The mitochondrial ATP synthase is a membrane protein complex that generates most of the ATP in eukaryotic cells. The translocation of protons through the membrane-bound Fo part, mediated by subunit a, drives the rotation of a membrane-embedded c-ring and the attached central stalk, which together form the rotor. The torque of the rotor against the stator subunits induces conformational changes in the (αβ)3 headpiece, thereby triggering catalysis. To reveal how the mitochondrial ATP synthase is modulated by lipids and organised into a dimer shaping discoid cristae in Euglenozoan mitochondria, we determined the structure of the ATP synthase dimer from E. gracilis.

The mitochondrial ATP synthase dimer was purified natively from E. gracilis and subjected to cryo-EM structure determination. The atomic model of the entire 2-MDa complex contains 29 different subunits (eight newly identified) and provides a comprehensive description of a markedly distinct mitochondrial ATP synthase dimer, including a previously unseen binding mode of its natural inhibitor protein IF1. The model of the complete mitochondrial ATP synthase contains 29 different proteins, of which 14 are phylum-specific, displaying a distinct architecture, particularly in the membrane region. The interactions between the monomers are expanded, resulting in a 45° dimer angle, compared to ~100° in yeast and mammals. Our atomic model of the E. gracilis mitochondrial ATP synthase shows that in contrast to yeast, subunits a, i/j, k do not contribute to the dimer interface, which instead is formed by species- and phylum-specific subunits and extensions of apparent homologs. The extensive dimer contacts are stacked across three layers: the matrix side, the transmembrane region and the lumenal side. Thus, despite the presence of conserved Fo subunits and the contribution to their extensions to the dimer interface, the E. gracilis mitochondrial ATP synthase displays a fundamentally different dimer architecture, when compared to the yeast, mammalian and Polytomella ATP synthases, suggesting that dimer formation evolved independently in different lineages. Our unsharpened map of the ATP synthase dimer with both monomers in rotational state-1 (IF1pointing towards the C2-axis), shows a continuous density from the C-terminus of IF1. This density extends towards the dimer interface and contacts the all-β-fold formed by subunits b and d, suggesting that also in Euglenozoa both F1 complexes in the ATP synthase dimer may be inhibited by a dimeric IF1. However, in contrast to the mammalian ATP synthase, the specific binding mode of the Euglenozoan IF1 assembly links two monomers within the dimer, rather than between neighbouring dimers.

>[2x]MTAVVKNLAKLPAATSQILTNVSKLQTFHGLLEERRDKYAPLAYHTYDNLKQKTTWHPIAHAWVDEGLPVSKKEYNEYCWLKKDMQRLLPLASPFVFGIYGILPLAVWLSNDGYLPSAFSSKKDIVSKKLEWYSSYGDDLRQQVGPMLQHRLKRHLRGTLNNEHRLMLDEVTESYKEIFYSHYTGQLRDVRKCAHLRLYDGTSTVLLLTNKEPVELTSELLQKWNAIKAAKLSPEEEKKARNEALIEAYKEQELHGGPHVKHMQGYGIPADTPLLGENAKGDQYTQPPESASIPLEQLEWTGDTVFIPAEYRTEMEDWGRELTKLANQFLLLPWRFVSNAWNQRRLVSWFEEILQEDALIAKEGGVQALSDDELKVALLDRAVIRCDEELTRGDMEARYKEISWLMSLRNPFIVLAWQTGYYRSTYSPEDDLPEASILPKLNRTVLDVDVHNELAPDHPEKPLPRVHPALYPNSHLALAKEVAVLAK;>[6x]MHYAEAATPAKSAGSAVAKKHLEAKQKIGFVHGIDGTIATIAPAASKVTVPYNTVLEIAVSATNIANALVFNLEKDGSIGVILLDNISEVRSGQDVYATGSLLKIPVGFHMLGKIINPLGKEIPTGLFTKAAPLLDDTKLGLVEEMAPNIVSRQPVNYNLLTGYKVIDTLIPVGRGQRELILGDRQTGKTSIALSTILNQTKVNNEILSKNNVLSVYVSIGQRCSNVARIHRLLTEYDAMKYCTIVAATAADPAGLQYLAPYAGTTLGEEFRNSGRHILLVYDDLSKQAVSYRQISLLLRRPPGREAYPGDVFYLHSRLLERSAMMSPQKGSGSLTSLPIVETLSNDVTAYIVTNVISITDGQIYLDAKLFTGGQRPAVNIGLSVSRVGSSAQNKAMKKVGGALKMLMGEYRKMAGEQTSGSQNVSPVMIRGARCLQLFNQKGPSYFMDAIVALYAVTNGYMDDVKLQYSKFYEFLLLNKDLPVLYGQVNNKYFYMYNKNLNYFIRYFGLNHEILEPELKKYIEIHTNLFLDNYQSRMNELKSDEDLVQLKNLLYACKRTV;>MVGRMMATAPATAADVKQVGYVQQIIGAVVDVTFTDSVPPVLTALTVDAKETGTLLTMEIVQHLDTKTARCICMSSTDMLRLRTPVVNTGSQITVPVGEATLGRIFNVMGDAIDQRGPVKNKVRWPIHRKAPTLAEQSGKDEVLVTGIKVIDLILPYCKGGKIGLFGGAGVGKTVIIMELINNVAKGHGGYSVFAGVGERTREGTDLYLEMMGSKVIDLQGDSKCVLVYGQMNEPPGARARVAQTALTMAEYFRDEAGQDVLLFVDNVFRFTQANSEVSALLGRIPAAVGYQPTLAEDLGMLQERITSTVKGSITSVQAVYVPADDITDPAPATTFSHLDATTVLSRSVAEAGIYPAVEPLECASRIMDPDAIDVNHYNVAMDIVEMLTKYKELQDIIAVLGIDELSEEDKLIVDRARKVAKFMSQPFAVAEVFTGMKGYYVQLEDCVSDFGSLLMGQCDNIPEMAFYMVGGLDSVKEKAAKMAAEAAAMRERARKAAEAK[6x];>[2x]MPGGGTIRFWREKLEGYKKYHQIVKTIKMVTLAKYRQTVVRTRVRDQTLRYTRKALDAKTQDDQEVIEKSECLLYVPITTNRGSCGALNTNMVRYLQEVENPKMTIISVGKKALDAMTKVFQDTYRRTILNDMKQAMSFQFAAYVLEHMNTVPWDRAQIVYNRYHGAASQKLAIFNLPKFEDWKQKLEEDSAGDGKIEEDGLLQSLPMKTALGELEETAVEDFYNFHSCLAVLNAVSENELSEYAARIVAVENQLGNITGLMQLADYTYNKTRKELITAELLEIIGTMTAMHAGKKVGLKKTEFWK;>[2x]MRASRTLLLSVSRFMRQDPRKFFPDNGFRFFDGPEDSFGDGNIPAQIILTLTRQDEFILKQEPVAAITIRTNEGEMGVLAGHEYTVQQLAPGILEVEYEGGKKDQYVISGGFAHVNDTGVVDINTVEAVPLEEIDHEKLAKALEEARAKSQSPDEAVRIQGEIALEIFEPLEAALH;>MSWRDAGISYLRYLSIVTRCIHEVQKEGPLLTKNVRFSTIGWKSLYLDHGATKEYTAIPAELEKIPENQVAQQHHA[2x];>MQKLSRVVCNRLVRFHGTVAASAGGKRYDLFGYEVSVATGPFIEEIKKAQFYDDAGEVIVKMNLANTPPDLQTYNAVLERILNCKSKRSQPVKGENKFAAMMDILEEMDARSGIKPNAESWGYVLKELVQAGDFRLGWVCIAGMKSLGITPDQALVDANEANAAKAKAAGTDFPAYLKKAAPESFDTKAWGI[6x];>MHMRRAVSVFGRCRSLNGLRNYAVPSPKYIEIYQSDFSRNAYPLELLGGSHVDFAKLLYSFADQVENKKFEVYVEDFKKLDSIIAEKGPFWAEEKIFQSPTFQGLSEGFKFILGWIQSEGAIDRLENVRLAYKELVNEARKETTATVIVAKEPSGNDLAEIRKQVEELHKESPLKDYKLVLETKVDPSIGGGYILEVCNQVVNRSAAAAAAETAALAKASAAQVDWTSLPAAPPRPSPSAPDTLIRLLGSVVDDLADADKVEQKYGA[2x];>MAAACAVRGFTTARPMLTPNKVKVPGRKPQDEEDLTWAEADRKLTPEERYARDKQMALLDKMTSQVEELEKSHTEQKKSNKGVKAQIEAISRQLEALKAQLKE[2x];>[20x]MQRGSSITKVVRRAALARSTRNAAIAYEVTVNGANLIGAGMAASGVGVPAIGVAMCFSSYMLAAARQPNMSAKLLPYCILGFALSEALALFTLLIALLELFVFS;>[2x]MAAKTIPFVASTALGERLFAGVQKVLAAAKAPVSLVQTDAKFAPADAKYLLAEPLSAAATGELANKYGLSSKVTSGAASQFYPNSIYPSLNVEVVQNLYALSNPAFSSLSATTTKAVTVKDESAIKLAELQKETERNISSFFRDEANKSVQATLRLACDKAIKTKADKKTVMVVTKPHGDAFDDLLAQVTKSESDGRADELRNSSVSVEPTLVGNAWPKLVMFPEGVNVVVCGPNASGDQVAQLFVGIAGGTGMVAQQLVGDAVVFTSANAEDNENPTGALLAASNLLTALGHEAEAKKIAAAVAKAYTTDRILPKELPGGKADLEAFIDAVAKHASA;>MFRGFRPVLAADAVKFQTLYNVLTGKQHLKDQVPVKDCNLTAIFGASWKADLNKWFDSEYAPKLPAAERDSAKKSLDLYLKRVDLTRYTREELTTYGILACGPGKVDALTEKHLLETGKARLEELTAGLGNKDEGVNAFRKEVEQEGKYANWPAEKSKALADKVIAASP[2x];>MTHAELHLFDLDEFMQTYKRLQTRQDWLIENKCKKSRLFSYVAAVIAFTVGKSATMSDEAILAKIDPYVTSEVRVQRGAWWRSGYFTKEEVEMMTPKGPIARYYKFLLGVRRFPLKHGALSWACGFVPAWLTFTSLNHWAQNRRLNRYLTQESVFGEMARELVRGKTADEATTSVMARVEKEILGVH[2x];>[2x]MSSYTGAALAPKSERLRLAFEEKQKDHQKCIEEAKGKGLKKDELIDACAWTHRKTILALKDWFAYRPPFQDRRSKWAEYCSIRHDSGSWLGWSQKFF;>MLNSNIYIIIYGGIIMYSIMIIIQMFLYNFSNKIYIEVEINKYILSKNNIDIYWIICNCTIIIIITTLNHIINKIGIYNMIEYNICYWLIGTGLGLYISPFIVFGYKFFVYIMDLNNYSLNIYHNNNKMNDIQQIYNGTNYNDTMIFFIKDINNIFTIYRSINFFMNWLYQMIYYGVRMWLVFVLHSFSLGSFGELITVITDNNLIFNVFYIGLLGLGFILYLIVIFYLGIQIYVYISFSLSFLHSTILLFLVNYIPHYNNKSIFNTFTNKSIY[2x];>[2x]MPSTSPADKDVPMSILHTHGLSYVNWCMSLAPGLLVFEGFFRARYYRSRVPPSRTVLMNGLKMRMFSLARQQAPKIVHKPVLSPIPEHLRLVKNVAQVQIDMLKLLNAQAAK;>MMRRACRIIRPSHVRGVSGVAPTIYLRSKAALPATSTTDVRPQLYALQRFAKAQLKTATEAERAAIEADIARYQEYLDSDLEKLKQDVAEDTAKKQKLIPLLDRYPDVPIEKIPEHANVLLKKIDACLEILSKDIGEVTDAEAHEMYFETSKFQILHIYTGCVASFPEGDVPPGAVECLPGQVIRTKVNGEDVMLEIDEVDPGYQVCWFKPDVPLPENAEILWSYPYEPTAALPTGTTWEEGQANVLIPAEPTPEAAVWPPTPVTNVYAPMAEKLALKSNPELKVLFKEALLQPAKLLPLDVDYQCSHDREVVEAKRDRYLTALVEAEQAPPLPFTPDVLQLQLEHNVLKGELIDRLRALEYTIVTEQLQARLHERRLRGDVIDEWEELDYHPLVRDDTYLAIDFGDPTFGRYIWKLFPHTDGDEECMFKDTRLDVLPPQVNPLNAILAQHTAQTPVHRSLEKRLWTEVRATAVSE[2x];>MAPLYPVLSQASLYKRHFFKNIKLFHVVFYVGAPCVTFGTAAWSGSNRNSREAIFMVIEERHGWDNFKKLSSHQQGVIMQEAAQESLLARNKGELHLP[2x];>MVYTNWQSSYTRLFVSKPWMWHPLAWMTLSVGIWWKFGKESLCNERSFYIHTHPKWAPHKFHTVYNWSRDPIKWTLAEQYASIIRNTNTDIEAVLKIKLPANAN[2x];>[2x]MAFGRTRPTLSSPLVPVWNDLRALQVFTSQEYMQKRGPGFTNTLEYKLSCLNPVKWYDMMKVMPGGKAFVGTALGLALFGGWGVEFVKNISVMTKEKPPIDWNNEKLGHLTRS;>LIPVSLVDLININIIFYILLLYTLLLFFIPLFLASINYTYHYIYKYYNYNYNFINNN[2x];>MSLAKVWMYASWIPRGIPKAMANELSSAAAALAHPEAIARVAQLESQGKNPYRVARAEFWQMYLACWPYRFRNTVVEWETCKAKVLKGSVDLQDIVDLLYLLAWAYLFWILGEIYGRGSLYGYRFDGEIHRQEAQNVILYKEKEAQEMAVVMEKLEKEIQEWLKTMEQE[2x];>[2x]MPLPNAVVQGYTSVRGPKRPLDHFYGRTPLNIDTLWHWVKFPHRYDNLRFAVCFWAFLVSAHFANKKQRNLRVEWEKNMEIQKKLHPSGLWSEEQAFAAAEKLGRPKAGHPMRVFEDGYQQFDLKPKLFDPDEEAHH;>MADHNKKDVGSWASPNEHLMFFDFSSWLLVDFGKRWERWVSFKKSFLTTTRSPYWSPQFFLLTFFQLRNSNVKLCENWNWAPKGDDFNLLHNSAAEPFGRDLKAHLEREAGAKHHH[2x];>[2x]MGGDAHAAPAEKPDPALDATKALPKALEEVEFFQSYAVRRKTGFHLFNRATGSPTIVGPMFYNLYNFVRIGRVSKYVCWLSLPLVFQRMWMKNRATGMEYDIDLENYAPFEAKKNPMHGH;>[2x]MSLPTFFLAPPLTEPFRARHRRKCIEKKDTFFQCLDKNKNETEPCEVEASGYSQECPDSWRRYFNEQRWKALELKGEVKHANLKNTQQHF;>[2x]MFGVTRKLLGELSEYVEVNEKGMPKPQALSLWNMPYAKRRALTKFARGVRWQFIVLFIALYNFKNRDDSHLLRRGAYN;>[2x]MMRISRKLLVPVANFRPKKPWDGPWGIQISQKKDRPFIAMWILFPLLLVDHLTREYYAYWHSSKVPVTDVFGDF;>[2x]MGGKASEAVTIAFRFPHRTTFLVKQNVGQKLNKGHQTFWQLVAGGWLFFLLINRTSFKPKLAAPKV>[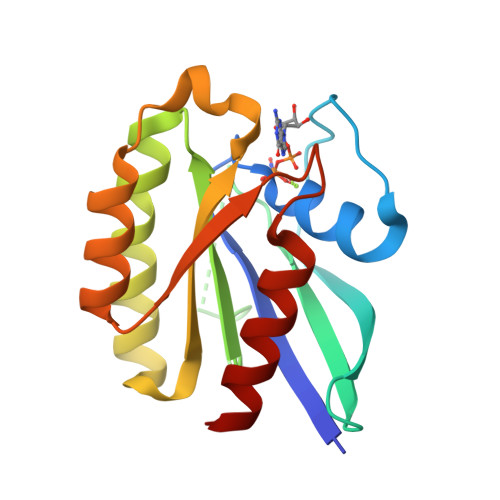4x]GSRAYSFKVVLLGEGCVGKTSLVLRYCENKFNDKHITTLGASFLTKKLNIGGKRVNLAIWDTAGQERFHALGPIYYRDSNGAILVYDITDEDSFQKVKNWVKELRKMLGNEICLCIVGNKIDLEKERHVSIQEAESYAESVGAKHYHTSAKQNKGIEELFLDLCKRMIET The Mycobacterium tuberculosis (Mtb) proteasome system selectively degrades damaged or misfolded proteins and is crucial for the pathogen’s survival within the host. Mtb 20S core particle features homoheptameric rings in a conserved α7-β7-β7-α7 configuration. These rings assemble to form three interconnected compartments: two antechambers formed by α7-β7 and a central degradation chamber. Stacked β-rings enclose the degradation chamber where active sites containing the catalytic triad of βT1, βD17, and βK33 proteolyze substrates.

We subsequently fit our molecular models to the first and last intermediate reconstructed maps and achieved excellent refinement statistics. Frames 1 and 20 represent the most distinct states in the continuum. The comparison between the initial and final frames clearly illustrates the transition from a disordered state to a well-ordered conformation that closely mirrors with the canonical resting state of the switch helices. Inspection of sequential frames highlights the progressive conformational changes of switch helix I and the decreasing flexibility of switch helix II that accompany the resting to auto-inhibited transition. Switch helix I significantly rearranges and moves towards switch helix II. Concurrently, residues 92-98 of switch helix II show increasing order, with their density becoming well-defined by frame 20, explaining the slower deuterium uptake of peptide β87-98.

>MSFPYFISPEQAMRERSELARKGIARAKSVVALAYAGGVLFVAENPSRSLQKISELYDRVGFAAAGKFNEFDNLRRGGIQFADTRGYAYDRRDVTGRQLANVYAQTLGTIFTEQAKPYEVELCVAEVAHYGETKRPELYRITYDGSIADEPHFVVMGGTTEPIANALKESYAENASLTDALRIAVAALRAGSADTSGGDQPTLGVASLEVAVLDANRPRRAFRRITGSALQALLVDQESPQSDGESSG[14x];>[14x]ATIVALKYPGGVVMAGDRRSTQGNMISGRDVRKVYITDDYTATGIAGTAAVAVEFARLYAVELEHYEKLEGVPLTFAGKINRLAIMVRGNLAAAMQGLLALPLLAGYDIHASDPQSAGRIVSFDAAGGWNIEEEGYQAVGSGSLFAKSSMKKLYSQVTDGDSGLRVAVEALYDAADDDSATGGPDLVRGIFPTAVIIDADGAVDVPESRIAELARAIIESRSGADTFGSDGGEK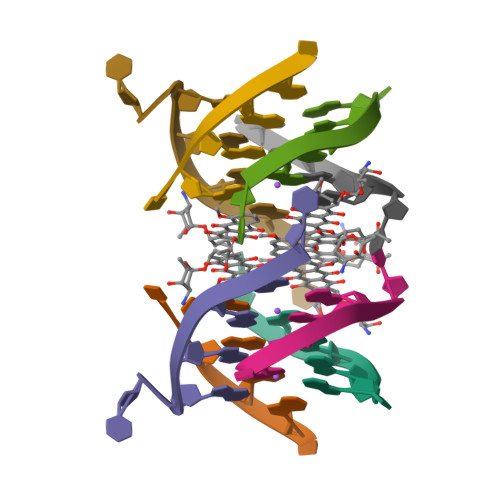>[4x]TGGGGT>[2x]GPLGSMSQSNRELVVDFLSYKLSQKGYSWSQMAAVKQALREAGDEFELRYRR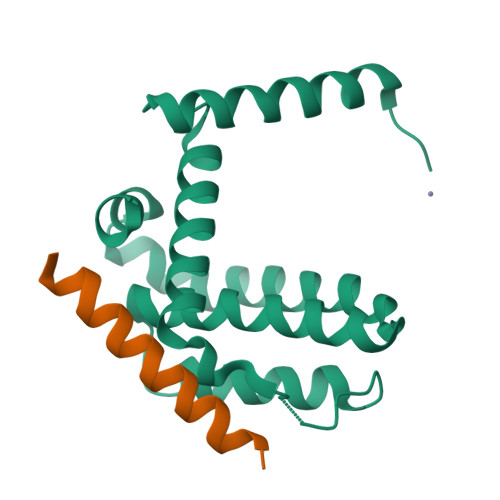AFSDLTSQLHITPGTAYQSFEQVVNELFRDGVNWGRIVAFFSFGGALCVESVDKEMQVLVSRIAAWMATYLNDHLEPWIQENGGWDTFVELYGNNAAAESRKGQER;>[2x]DMRPEIWIAQEFRRIGDEFNAYYARR> SMVQSSGPMDVTSLTEELK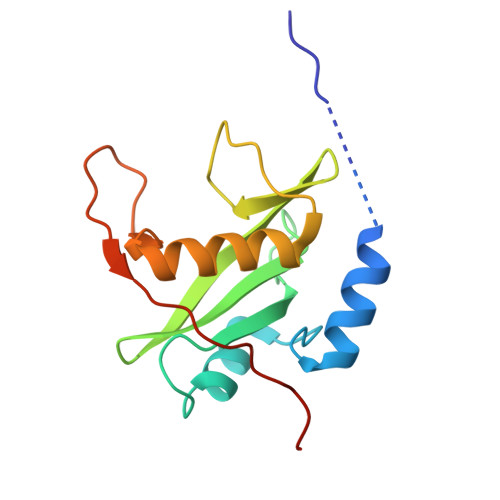KLAKQGWYWGPITRWEAEGKLANVPDGSFLVRDSSDDRYLLSLSFRSHGKTLHTRIEHSNGRFSFYEQPDVEGHTSIVDLIEHSIGDSENGAFCYSRSRLPGSATYPVRLTNPVSRFMQVRS> AAECTVPIGWSEPVKGLCKARFTRYYCMGNCCKVYE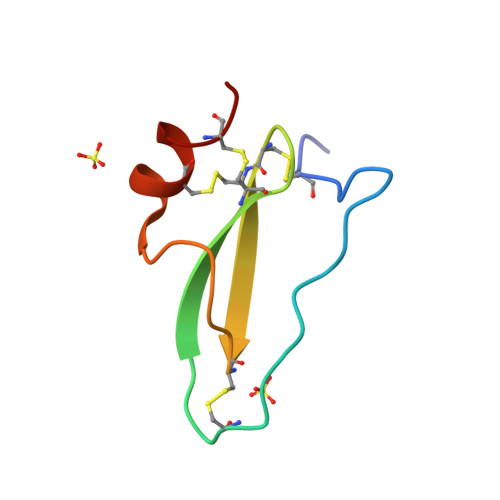GCYTGGYSRMGECARNCPG> DNEEDIDVILKKSTILNLDINNDIISDISGFNSSVITYPDAQLVPGINGKAIHLVNNESSEVIVHKAMDIEYNDMFNNFTVSFWLRVPKVSASHLEQYGTNEYSIISSMKKHSLSIGSGWSVSLKGNNLIWTLKDSAGEVRQITFRDLPDKFNAYLANKWVFITITNDRLSSANLYINGVLMGSAEITGLGAIREDNNITLKLDRCNNNNQYVSIDKFRIFCKALNPKEIEKLYTSYLSITFLRDFWGNPLRYDTEYYLIPVASSSKDVQLKNITDYMYLTNAPSYTNGKLNIYYRRLYNGLKFIIKRYTPNNEIDSFVKSGDFIKLYVSYNNNEHIVGYPKDGNAFNNLDRILRVGYNAPGIPLYKKMEAVKL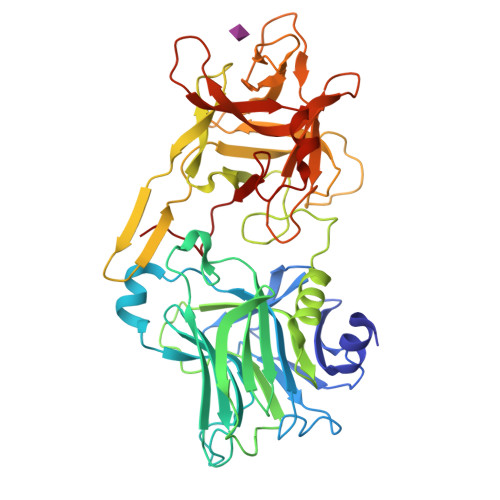RDLKTYSVQLKLYDDKNASLGLVGTHNGQIGNDPNRDILIASNWYFNHLKDKILGCDWYFVPTDEGWTND[(2~{R},3~{R},4~{R},5~{R})-2-[8-[3-[[(2~{R},3~{S},4~{R},5~{R})-5-(6-aminopurin-9-yl)-3,4-bis(oxidanyl)oxolan-2-yl]methyl-methyl-amino]prop-1-ynyl]-6-azanyl-purin-9-yl]-5-(hydroxymethyl)-4-oxidanyl-oxolan-3-yl] 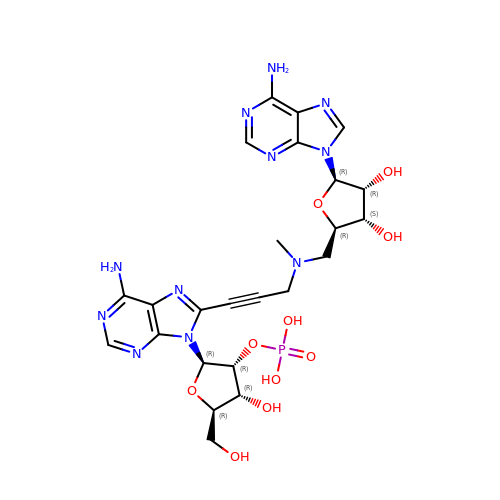dihydrogen phosphate | C24 H30 N11 O10 P | LZWZGJMZXMPLGZ-KRSQEUQLSA-N> MDKATLVKTIAYRMGNVKGQDTAIDFELALSIERLEGQE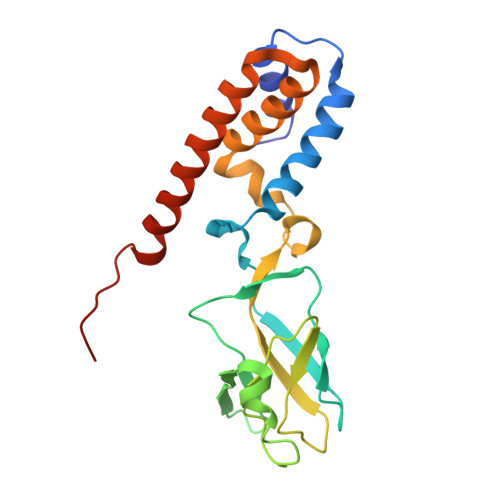FVPWFLLSENNFFEGTAQENRIPVPRGFIREYEEGSLYLRRVAGTGKCLIKKSQDQLLKYEGMTGEPSHYSLTNQYFRIYPVPQEDFKVELLFYRKSSTLNVEDNPWYEYAAELLVAETIWAMLSARRDKMADYWKSVAADQMRRLTILDAERRLANQEIFMG>DLPRHIAVLCDGNRRWARSAGYDDVSYGYRMGAAKIAEMLRWCHEAGIELATVYLLSTENLQRDPDELAALIEIITDVVEEICAPANHWSVRTVGDLGLIGEEPARRLRGAVESTPEVASFHVNVAVGYGGRREIVDAVRALLSKEL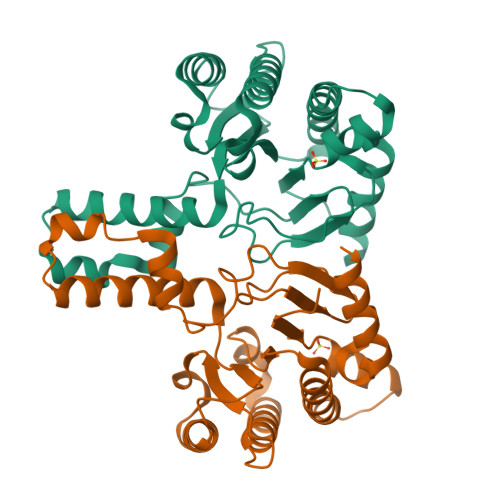ANGATAEELVDAVTVEGISENLYTSGQPDPDLVIRTSGEQRLSGFLLWQSAYSEMWFTEAHWPAFRHVDFLRALRDYSAR[2x]> MWGNLWTEASYQLNFNIGFSSLRSDVLIHLAQWQYWWWFWFALIWSFYYFIILKVARFRVLKMRPKISTSYRPHGKWGDFLACIIPLIWCINILTNSNLILRLIEWQNESSLFTVRVRARQWYWIYKFELKNFTDILSTPKNIGNNRWQINTFGELQTADDYLHVLQLRSQNKWVKNYWNRSLQETGKTNKAHVISPQEQLRLSLINQYKSLNLSSSIKHNAPFINRDLYVFDDLFSYNLGDITTKKSLFNDKNSFLTSYSYLNNNSWNNNEFDLIDNLPFTTLFDNNDLFNNYKSFFQDSIFNSPKKQLSSDSKQLFKHIIYRSIKNNIIQDYTKLVKHEDFDEYSRWIKRSPGEVLPLRIIKYPLGLETIHNNIFENTNNEGNVELFRLRFNSNSSKMQHKLVQDTIYLTLKQKRYNRK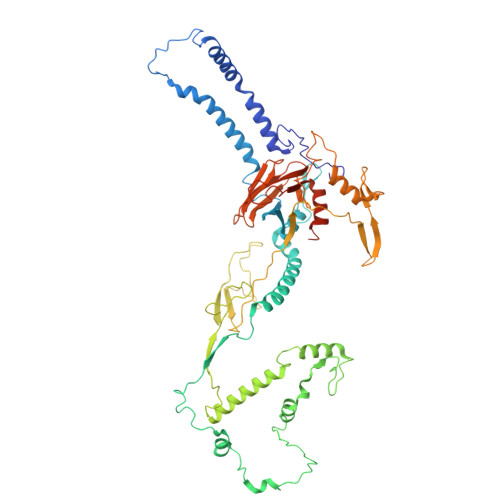KVVAPQIKYYKDDNGNKTDLVKYTGKPYLSNDKLLKQSIYDQTTQYKLIKKNKKRGELIPVTLARRILRTKKTLVLPAHVNITLITNSYDIVHSWFIPGLGIKLDCVPGRSTHHTFFIDNVGFYYGQCAEICGRYHHHMPIRVCALPFEHFLLWWNTFGLPKMLNTVSRKRFETHYELRKYSW> MGSSNTVTSAVKTQYVEIESVMGFYFNTEDKFDTAQIKKAVLHTVYNEGYTGDDGVAVVLREYESEPVDITAELTFGDATPANTYKAVENKFDYEIPVYYNNATLKDAEGNDATVTVYIGLKGDTDLNNIVDGRDATATLTYYAATSTDGKDATTVALSPSTLVGGNPESVYDDFSAFLSDVKVDAGKELTRFAKKAERLIDGRDASSILTFYTKSSVDQYKDMAANEPNKLWDIVTADAEEE;> SSVTADLNNAVINVDEMNEAFKDVPDLEGEGAHITL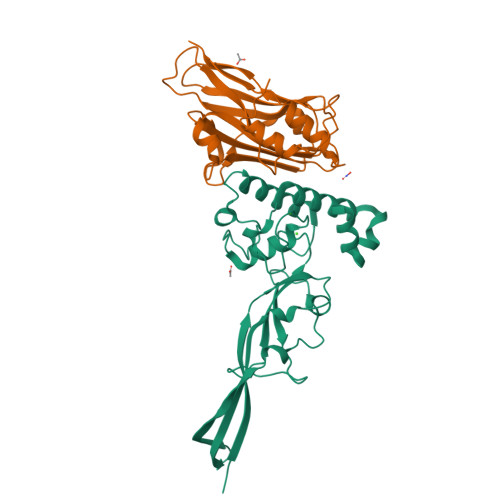SNTTAKPGEMAEVTMSVSNADMQWNMCGIHIIYPDILKPEMKDPEERTVAFQKGDALEAATGIVCMEWQEGLPPVLTENKKGCLFLTAMFSGNQGGEGDMATFRFKVPDNAEPGAVYNLGYYYMNTDLFINEQNIPTYQKYAFTHMEGGTITVEL>MENQIKANTKKEYDEWFKPYAEKTHLKSVLTNSASFCDALPDLSIFEVKMGLATDDREKDSIYACAMVEATKFCAPIYECGWACCTGMVENGLKWFDKNKDVIKLWDGKYSDLMKNVPEPEQLVAYQRAAQKWRQDNKFEINQYTRSLTHSVQADYKVPGEYAVEVKEMLSDMVRRRNILLNGNGDDAGKKGPVSREHVNWGRELAAGKFQVVFNPPWGDINKTGRSGIPLAVTSMVKVAELDGHKRLEDIRKTLLDLKKWIEDNKDELEDGKGDELVKTLTKQLADAIELAKKSSALRAQGAQIDSIFSSYYWAWKAGITPVTFPTLSQFLFEMGQGPRGGKKMIKALTNTPLKWGKKIISLFAEDDFNGNKLY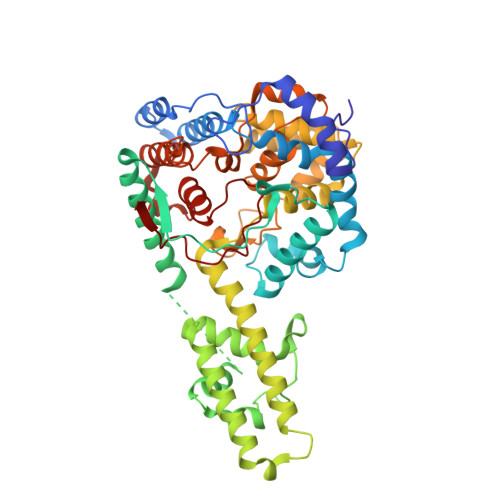MHPGVLTAGRMSEMGACFGVVPVSNPEDAVLGSGHSKSLLNYKIDTNAGNPCAKEIVQLFRIQKAGFDLDSMDIVASEHLLHQSLVGKRCHFQNAYKVKGNATNVEIV[2x]>[12x]MSSTPSNQNIIPIIKKESIVSLFEKGIRQDGRKLTDYRPLSITLDYAKKADGSALVKLGTTMVLAGTKLEIDKPYEDTPNQGNLIVNVELLPLAYETFEPGPPDENAIELARVVDRSLRDSKALDLTKLVIEPGKSVWTVWLDVYVLDYGGNVLDACTLASVAALYNTKVYKVEQHSNGISVNKNEVVGKLPLNYPVVTISVAKVDKYLVVDPDLDEESIMDAKISFSYTPDLKIVGIQKSGKGSMSLQDIDQAENTARSTAVKLLEELKKHLGI;>[12x]MREMLQVERPKLILDDGKRTDGRKPDELRSIKIELGVLKNADGSAIFEMGNTKAIAAVYGPKEMHPRHLSLPDR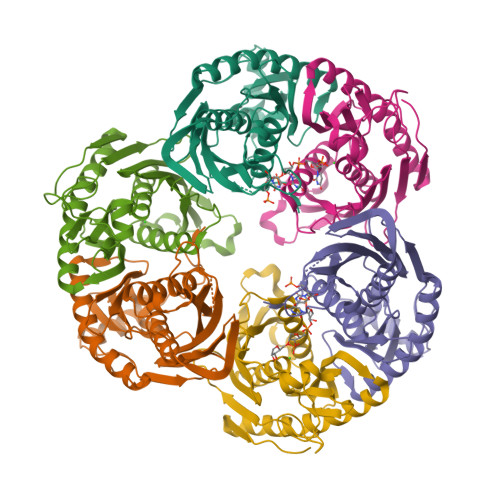AVLRVRYHMTPFSTDERKNPAPSRREIELSKVIREALESAVLVELFPRTAIDVFTEILQADAGSRLVSLMAASLALADAGIPMRDLIAGVAVGKADGVIILDLNETEDMWGEADMPIAMMPSLNQVTLFQLNGSMTPDEFRQAFDLAVKGINIIYNLEREALKSKYVEFKEEGV>GGG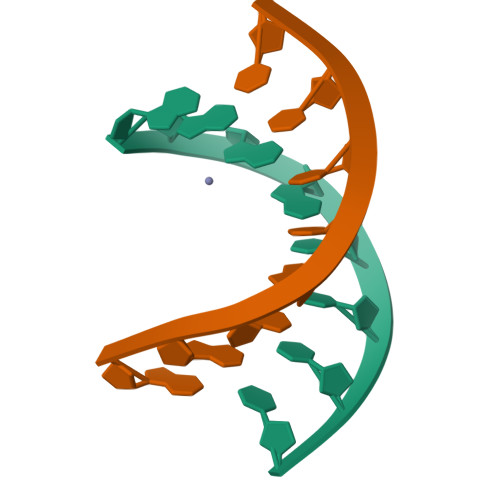ATCCC[2x]> GAMGMPSLKDEVSFENRVAETHKIRSKYPNRIPVVIERANRSNLPIIEKKKFLVPMNMLVGEFKFILHQHINQSAYGSNMKLFRERTIYLFVNNIVPKTGLLMQ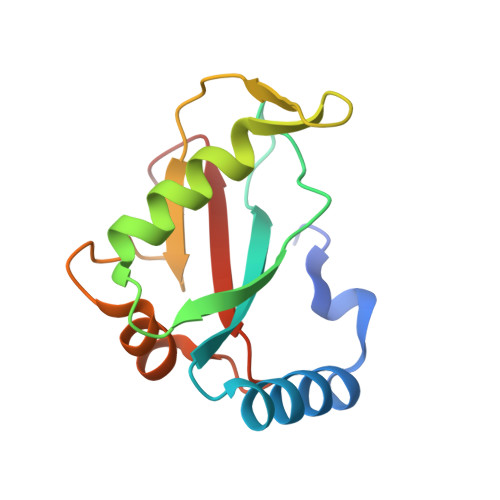DLYEMYKDEDGYLYMEYSSESSLG>GAMAE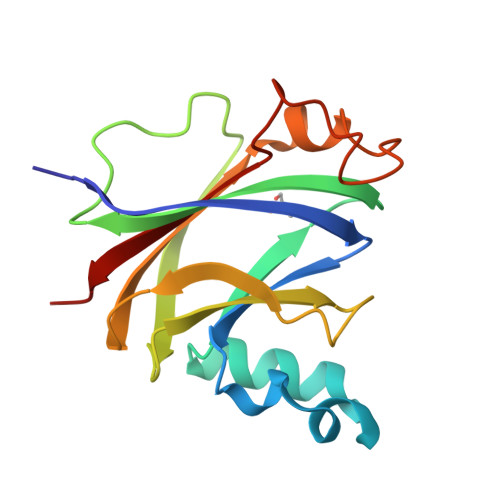EVAEIILPASTWILFFDASCSINSPAFWSTNDAVDRIWRLKIAHELVLLQVVLEGYFKVRCILRSSAPAFEMVNADVSELVSIVLPSGRLVACTTDEPTLNRHVLTVPPGRYRVLREWSVHEESKHYDVESAEAYPADEGPDGIITLWPER[3x]>[2x]GSSESFKDAATEKFRSASVGAEEYMYDQTSSG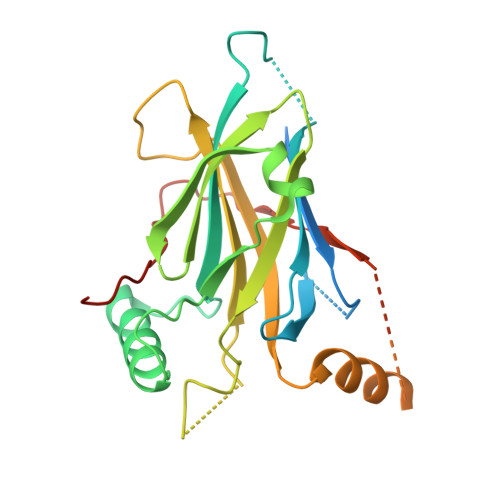TFQYTLEATKSLRQKQGEGPMTYLNKGQFYAITLSETGDNKCFRHPISKVRSVVMVVFSEDKNRDEQLKYWKYWHSRQHTAKQRVLDIADYKESFNTIGNIEEIAYNAVSFTWDVNEEAKIFITVNCLSTDFSSQKGVKGLPLMIQIDTYSYNNRSNKPIHRAYCQIKVFCDKGAERKIRDEERKQNRKKGKGQASQTQCNSSSDGKLAAIPLQKKSDITYFKTMPDLHSQPVLFIPDVHFANLQR>[3x]QDVRVRVLPEVRGRLGGTVELPCHLLPPTTERVSQVTWQRLDGTVVAAFHPSFGVD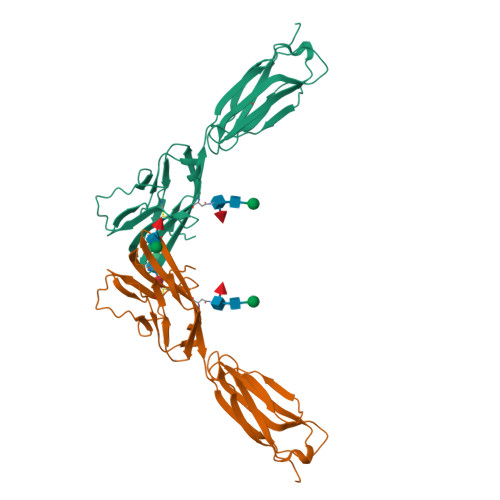FPNSQFSKDRLSFVRARPETNADLRDATLAFRGLRVEDEGNYTCEFATFPNGTRRGVTWLRVIAQPENHAEAQEVTIGPQSVAVARCVSTGGRPPARITWISSLGGEAKDTQEPGIQAGTVTIISRYSLVPVGRADGVKVTCRVEHESFEEPILLPVTLSVRYHHHHHH>[2x]MNNPADAGINLNYL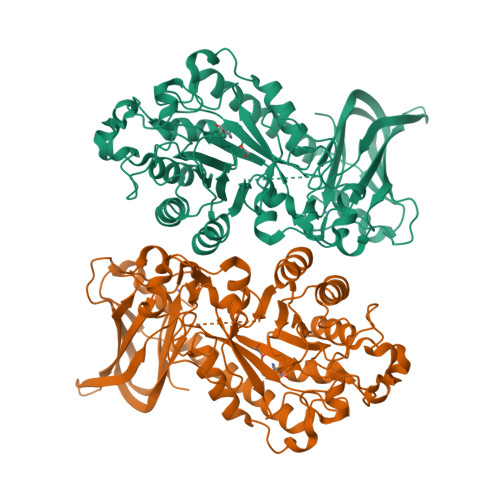ANVRPSSRQLAWQRMEMYAFLHFGMNTMTDREWGLGHEDPALFNPRNVDVDQWMDALVAGGMAGVILTCKHHDGFCLWPSRLTRHTVASSPWREGKGDLVREVSESARRHGLKFGVYLSPWDRTEESYGKGKAYDDFYVGQLTELLTQYGPIFSVWLDGANGEGKNGKTQYYDWDRYYNVIRSLQPDAVISVCGPDVRWAGNEAGHVRDNEWSVVPRRLRSAELTMEKSQQEDDASFATTVSSQDDDLGSREAVAGYGDNVCWYPAEVDTSIRPGWFYHQSEDDKVMSADQLFDLWLSAVGGNSSLLLNIPPSPEGLLAEPDVQSLKGLGRRVSEFREALASVRCEARTSSASAAAAHLVDGNRDTFWRPDADDAAPAITLTLPQPTTINAIVIEEAIEHGQRIEHLRVTGALPDGTERVLGQAGTVGYRRILRFDDVEVSSVTLHVDGSRLAPMISRAAAVRI>GPLLKLFDISILPKSGEPKLFLPVPSLPCQEAEKTNDKYVLAMAQRAMHDVPISSKQLTANLLPVKFKPLLSIVRYTPNYYYWVSMRKETIASANLCTVAAFLDESLCWGQQYLKNDFIFSENGKDIILDTSSALLSQLVHKIKMLPFCHCLMQTTPQDHIVKQVCYLIASNNRILDAVRYLQTSVIKSPIVLLLAYAVCLPAAIICTKNETQLYSHCMRILKEYRPGDVMNILHESLTQHLNKCPSSTCAYTTRAIVGTKANTTGLFFLPTQ[2x]

KSHV also expresses several early proteins including ORF57 (Mta), a member of the conserved multifunctional ICP27 protein family, which is essential for productive replication. ORF57/Mta interacts with PAN RNA via a region termed the Mta responsive element (MRE), stabilizing the transcript and supporting nuclear accumulation. We also obtained the high-resolution structure of the C-terminal IHD from hvsORF57 in both the presence and absence of a PAN RNA MRE oligonucleotide fragment. The C-terminal IHD of hvsORF57 forms a compact homo dimer, approximately 65  ×  60  ×  40 Å.

In order to investigate the 3D structure of an ORF57 C-terminal IHD experimentally, first we purified the hvsORF57Δ146 and ksORF57Δ153 protein constructs in the absence of RNA and screened with a variety of crystallization conditions using six commercial screens (SG1, JCSG+, PACT Premier, BCS, LMB and Morpheus; Molecular Dimensions). However only the hvsORF57Δ146 construct produced diffracting crystals. Initial phases were obtained from single wavelength anomalous dispersion (SAD) experiments carried out on selenomethionine derivatized crystals in Phenix.AutoSol. Model building and refinement were carried out against the same data, extending to a resolution of 1.86 Å. Each polypeptide chain is composed of 11 α-helices and a small β-sheet formed by two parallel strands, folded into an individual globular domain. One CHCC zinc finger is formed by each chain from residues C293, H385, C389 and C394, which coordinate a zinc ion in a tetrahedral geometry. Residues 181–417 form the globular folded core domain preceded by residues 146–180, which comprise an extended N-terminal arm largely lacking secondary structure that domain swaps, wrapping around the dimeric partner's globular domain. The major homo-dimer interface is linear and formed by contacts between α-helices 3, 5 and 11 which lie approximately parallel to each other making symmetric contacts and forming a groove. The groove is bridged by α-helix 6, where residues Y311 and S315 from separate polypeptide chains contact each other, with the sidechain hydroxyl oxygens of the Y311 pair distanced by 2.6 Å. Analysis of the surface electrostatic distribution indicated that the groove has a net positive charge.> MALTQSVGGDSSADRLFPPQWICCDIRYLDVSILGKFAVVMADPPWDIHMELPYGTLTDDEMRRLNIPVLQDDGFLFLWVTGRAMELGRECLNLWGYERVDEIIWVKTNQLQRIIRTGRTGHWLNHGKEHCLVGVKGNPQGFNQGLDCDVIVAEVRSTSHKPDEIYGMIERLSPGTRKIELFGRPHNVQPNWITLGNQLDGIHLLDPDVVARFKQRYPDGIISKPKNL;> GSLKGTQSLNPHNDYCQHFVDTGHRPQNFIRDVGLADRFEEYPKLRELIRLKDELIAKSNTPPMYLQADIEAFDIRELTPKFDVILLEPPLEEYYRETGITANEKCWTWDDIMKLEIDEIAAPRSFIFLWCGSGEGLDLGRVCLRKWGYRRCEDICWIKTNKNNPGKTKTLDPKAVFQRTKEHCLMGIKGTVKRSTDGDFIHANVDIDLIIT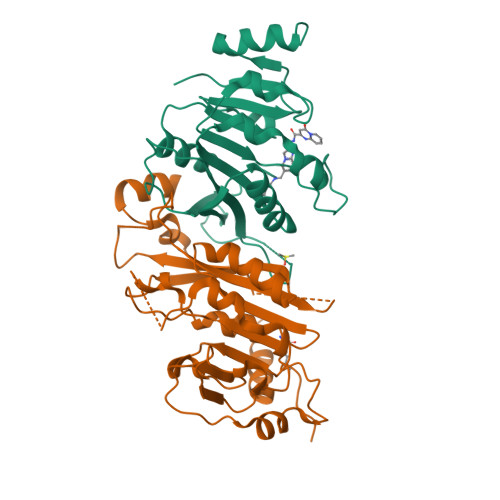EEPEIGNIEKPVEIFHIIEHFCLGRRRLHLFGRDSTIRPGWLTVGPTLTNSNYNAETYASYFSAPNSYLTGCTEEIERL>[2x]PLGSRYEDAYQYQNIFGPLVKLEADYDKKLKESQTQDNITVRWDLGLNKKRIAYFTLPKTDSDMRLMQGDEICLRYKGDLAPLWKGIGHVIKVPDNYGDEIAIELRSSVGAPVEVTHNFQVDFVWKSTSFDRMQSALKTFAVDETSVSGYI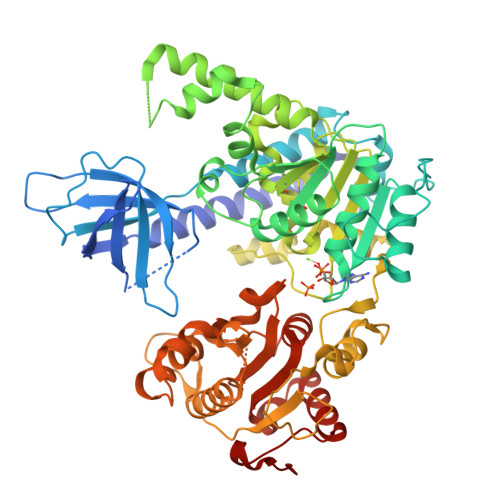YHKLLGHEVEDVIIKCQLPKRFTAQGLPDLNHSQVYAVKTVLQRPLSLIQGPPGTGKTVTSATIVYHLARQGNGPVLVCAPSNIAVDQLTEKIHQTGLKVVRLCAKSREAIDSPVSFLALHNQIRNMDSMPELQKLQQLKDETGELSSADEKRYRALKRTAERELLMNADVICCTCVGAGDPRLAKMQFRSILIDESTQATEPECMVPVVLGAKQLILVGDHCQLGPVVMCKKAAKAGLSQSLFERLVVLGIRPIRLQVQYRMHPALSAFPSNIFYEGSLQNGVTAADRVKKGFDFQWPQPDKPMFFYVTQGQEEIASSGTSYLNRTEAANVEKITTKLLKAGAKPDQIGIITPYEGQRSYLVQYMQFSGSLHTKLYQEVEIASVDAFQGREKDFIILSCVRANEHQGIGFLNDPRRLNVALTRARYGVIIVGNPKALSKQPLWNHLLNYYKEQKVLVEGPLNNLRESLMQFS> MPDFLGHAENPLREEEWARLNETVIQVARRSLVGRRILDIYGPLGAGVQTVPYDEFQGVSPGAVDIVGEQETAMVFTDARKFKTIPIIYKDFLLHWRDIEAARTHNMPLDVSAAAGAAALCAQQEDELIFYGDARLGYEGLMTANGRLTVPLGDWTSPGGGFQAIVEATRKLNEQGHFGPYAVVLSPRLYSQLHRGGEIETIRQLASDGVYQSNRLRGESGVVVSTGRENMDLAVSMDMVAAYLGASRMNHPFRVLEALLL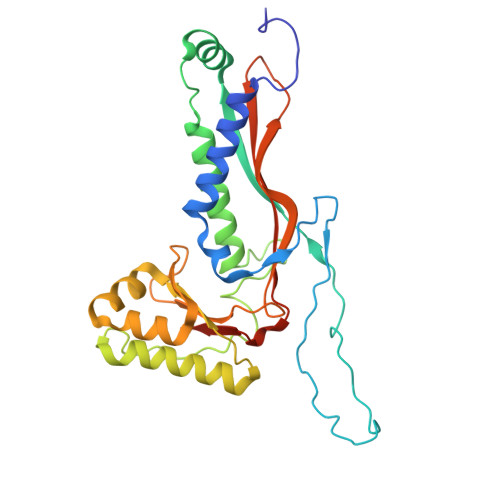RIKHPDAICTLEGAGATERR>[2x]GPLGSPEFQRTKPFSVPNIPMNLMSNSRVPMLIDGMMVSNDQNQVPQFQNGRVTLDGQLQGTTTVSAACIARMRGRIFNNNGNYGVNLAELDGNPYHAFDSPAPLGFPDFGNCDLHMTFVKINPTELSTGDPSGKVVIHSYDATFAPHLGTVKLEDNNELDQFVGKEVVLELTWVSNRTGATLNLWAVPNYGSNLTQASQLAPPIYPPGFGEAIVYFTSTFPTVSNPKVPCTLPQEFVSHFVNEQAPTRGDAALLHYVDPDTHRNLGEFKMYPEGYMTCVPNAGGGPQTLPINGVFVFISWVSRYYQL

NoV VP1 has two principle domains, the shell (S) and the protruding (P) domains, linked by a short, flexible hinge. The S domain builds the interior shell that forms the basic structure of the icosahedral capsid, while the P domain dimerizes constituting the arch-like protrusions extending from the shell. HuNoVs recognize histo-blood group antigens (HBGAs) as attachment factors or receptors which play an important role in the host susceptibility to huNoV infections. BV, a clinical isolate, bound uniquely to the Le, but not the A and H antigens, making the BV distinct from other tested GI NoVs that bind generally the A and H antigens.

In this study, the crystal structures of the BV P dimers in complex with the type 1 Leb and the type 2 Ley antigens, respectively, were resolved. The BV P dimers in complex with type 1 Leb and type 2 Ley tetrasaccharides, respectively, were crystallized in the same space group and unit cell dimension of native protein and thus may be viewed as isomorphous with the native crystal. Fourier difference maps were calculated from diffraction intensity Fcomplex − Fnative combined with phase angle derived from final native protein structure, which unambiguously reveals the high resolution electron density maps of the bound tetrasaccharides. Two symmetric HBGA binding interfaces are identified on the top of the BV P dimer at the common boundary between the two P monomers, sharing similar locations with the other three known GI binding interfaces. The conformational binding interface of BV is composed of two major areas, a β-Gal binding site and a Le epitope binding site, formed by ten amino acids from 3 (P-, T-, and S-) loop regions. The β-Gal of the precursor makes a major contact with the “bottom” of the binding interface, which is stabilized by residue T397, while the Le epitope, the α-1,3/4 Fuc (Le Fuc), contacts with another part of the “bottom” and is stabilized by the other “wall” (S346′, T347′, G348′ and D349′) to support the binding outcomes. In fact, BV does not form a single H bond with the H epitope in binding to the type 2 Ley antigen, while only one water mediated H epitope between D349′ of the P-loop and the H epitope was seen in BV binding to the type 1 Leb antigen. Finally, BV also forms a water mediated H bond with the N-acetyl glucosamine (GlcNAc) of the precursor through T347′ of the P-loop in binding to the Leb antigen, a scenario that has not yet been observed in the other three GI NoVs. In fact, the H epitope of the Leb and Ley antigens played a minor role in the binding outcomes as it does not at all participate in binding to Ley, or interacting with the Leb through a single H bond among the eleven H bonds in total.> GSHMDYLVTEEEINLTRGPSGLGFNIVGGTDQQYVSNDSG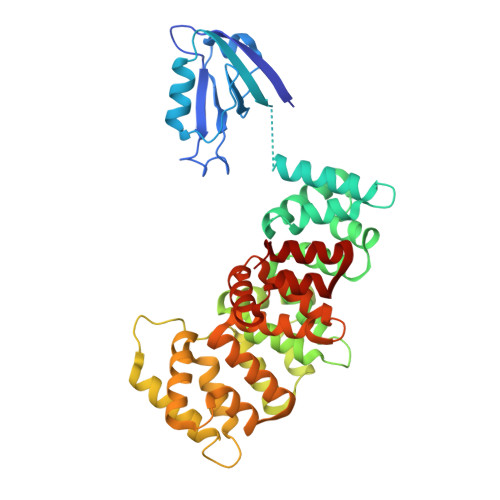IYVSRIKENGAAALDGRLQEGDKILSVNGQDLKNLLHQDAVDLFRNAGYAVSLRVQHRLQVQGSAYTNFDAERDALNIETAIKTKGVDEVTIVNILTNRSNEQRQDIAFAYQRRTKKELASALKSALSGHLETVILGLLKTPAQYDASELKASMKGLGTDEDSLIEIICSRTNQELQEINRVYKEMYKTDLEKDIISDTSGDFRKLMVALAKGRRAEDGSVIDYELIDQDARDLYDAGVKRKGTDVPKWISIMTERSVPHLQKVFDRYKSYSPYDMLESIRKEVKGDLENAFLNLVQCIQNKPLYFADRLYDSMKGKGTRDKVLIRIMVSRSEVDMLKIRSEFKRKYGKSLYYYIQQDTKGDYQKALLYLCGGDD>GSKKRRRRRPEPQLKGIVTKLYSRQGYHLQLQADGTIDGTKDEDSTYTLFNLIPVGLRVVAIQGVQTKLYLAMNSEGYLYTSELFTPECKFKESVFENYYVTYSSMIYRQQQSGRGWYLGLNKEGEIMKGNHVKKNKPAAHFLPKPLKVAMYKEPSLHDLTEFSRSGSGTPTKSRSVSGVLNGGKSM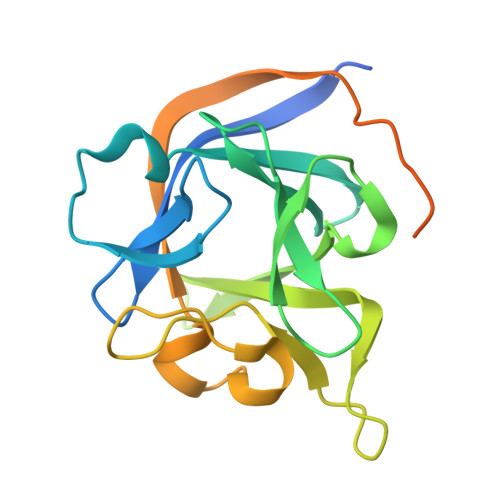SHNEST[2x]>MDRPVRVLFVCLGNICRSPMAEGIFRKLLKERGLEDRFEVDSAGTGAWHVGEPMDPRARRVLEEEGAYFPHVARRLTREDVLAYDHILVMDRENLEEVLRRFPEARGKVRLVLEELGGGEVQDPYYGDLEDFREVYWTLEA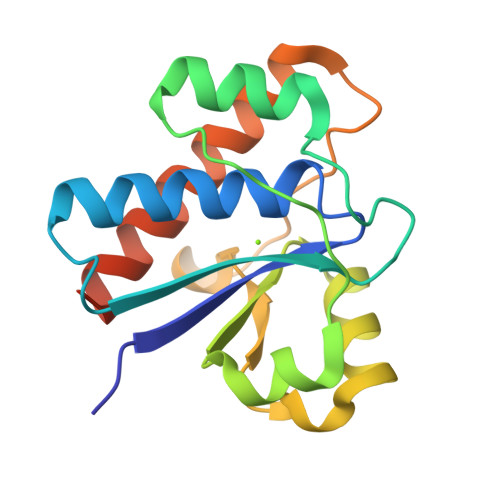ALQAFLDRHGSPSPAAEGRA[4x]>[2x]SIIRPQLKFREKIDNSNTPFLPKIFIKPNAQKPLPQALSKERRERPQDRPEDLDVPPALADFIHQQRTQQVEQDMFAHPYQYELNHFTPADAVLQKPQPQLYRPIEETPCHFISSLDELVELNEKLLNCQEFAVNLEHHSYRSFLGLTCLMQISTRTEDFIIDTLELR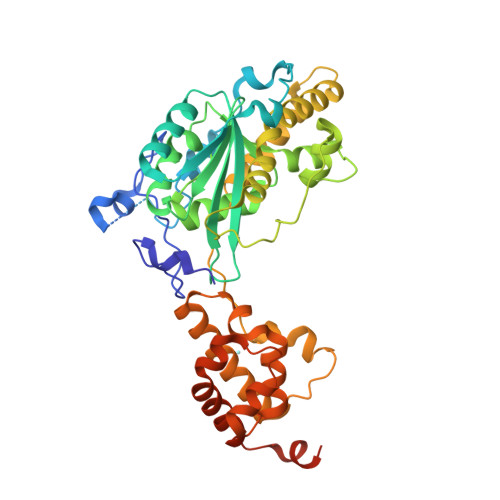SDMYILNESLTDPAIVKVFHGADSDIEWLQKDFGLYVVNMFDTHQAARLLNLGRHSLDHLLKLYCNVDSNKQYQLADWRIRPLPEEMLSYARDDTHYLLYIYDKMRLEMWERGNGQPVQLQVVWQRSRDICLKKFIKPIFTDESYLELYRKQKKHLNTQQLTAFQLLFAWRDKTARREDESYGYVLPNHMMLKIAEELPKEPQGIIACCNPVPPLVRQQINEMHLLIQQAREMPLLKSEVAAGVKKSGPLPSAERLENVL> MTQTAAKSLKFPKDFLWGAATAAYQIEGAANEDGRGPSIWDTFSHTPGKVHNGDNGDVACDHYHRYKEDVELMKELGLNAYRFSISWPRILPEGEGKVNQKGLDFYNNLIDELLENGIEPFVTLYHWDLPQALQDKGGWENRETVDAFAEYARVCFERFGDRVKYWITFNEPNVFAVLGYLSGVHPPGMKDLKKAFRAAHNLLLAHARAVKAYREISQNGQIGITLNLSPVYPASDNEEEDKAAAERADQFNNWFLDPIFKGKYEHMLERLGEQIAANGGELPEITDEMEILSASLDFIGLNYYTSNLVRANPNS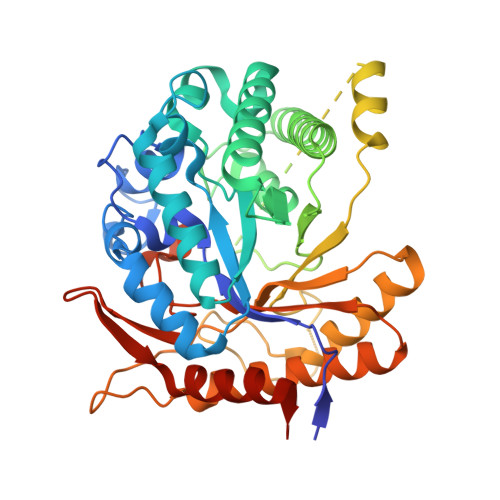GSSSVKPPDLPRTDMGWEIYPEGLYDLLKRIHEKYNLPIYITENGMAVDDEVEDGAVHDTNRIDYLKEHLEAVHKAIEEGVNVRGYFVWSLMDNFEWANGYSKRFGLIYVDYKTQKRTPKKSAYWYREVIKSNGLELEHHHHHH>[2x]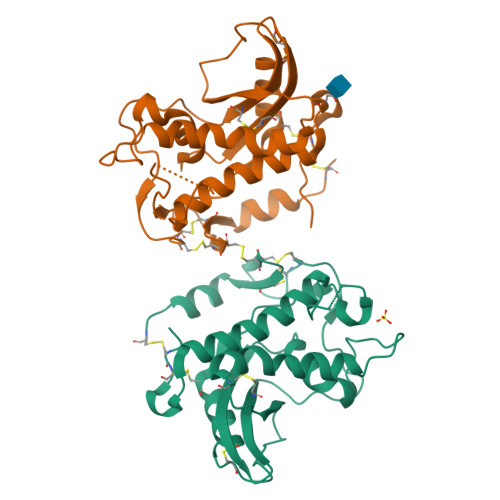EAEAGFCCPADLNQTDEARKIFLDFHNQVRRDIAGASPLLNLTGAVQMRNVLGPAKNMYRMDWDCNLEAKAKAMIWPCTTPLPIDTSIPQNLAQWLLFQNSQENEVLTQTPWSWVTASLRNLQPDTEANIYNWQIRPLSNIANWQNLKVGCAHKVCKFPTGTNMVVSCAYGGEVLQDNEVVWDKGPTCMCNAYPNSFCCNNLCDTIAAATLRNQPCKST For instance, the U5 snRNP 200 kDa helicase (SNRNP200; Brr2p in yeast) unwinds the initially extensively base-paired U4 and U6 snRNAs during spliceosome activation and releases U4 snRNA and all U4/U6-associated proteins, necessitating re-assembly of the U4/U6 di-snRNP and the U4/U6-U5 tri-snRNP after splicing. SNRNP200 comprises an auto-regulatory N-terminal region (residues 1–394), followed by a helicase region (residues 395–2129; SNRNP200HR) composed of tandem helicase cassettes (N-/C-terminal cassette, NC/CC). Both helicase cassettes comprise dual RecA-like NTPase domains, a winged helix (WH) domain, a helical bundle (HB) domain, a helix-loop-helix (HLH) domain and an immunoglobulin-like (IG) domain. Only the N-terminal cassette (residues 395–1324; SNRNP200NC) is an active ATPase/RNA helicase, while the C-terminal cassette (residues 1282–2136; SNRNP200CC) is catalytically inactive and serves as an intra-molecular regulator of the NC helicase activity.

We have previously characterized the interaction of SNRNP200 with two splicing factors that are also largely intrinsically disordered, FBP21 and C9ORF78 (34,35). FBP21 enters the spliceosome during formation of the pre-catalytic B complex together with seven additional B-specific proteins and leaves the spliceosome again during the following activation step, likely facilitating ordered transitions toward a catalytically competent spliceosome. Like TSSC4, both proteins also contact the SNRNP200 CC. Notably, the binding site of TSSC4 binding region 4 (residues 303–318) overlaps with a binding site of FBP21 and C9ORF78 regions at the Sec63 unit of the SNRNP200 CC. Moreover, all three proteins employ an F-R (F315-R316 in TSSC4; F8-R9 in C9ORF78) or L-R (L369-R370 in FBP21) motif to engage in similar contacts with the F1983, E1944 and E2119 residues of SNRNP200HR. This observation supports the idea that the SNRNP200 CC serves as a latching point for diverse intrinsically disordered proteins (IDPs) that either function during snRNP assembly (TSSC4) or during different stages of the splicing cycle (FBP21, C9ORF78). Mutually exclusive binding of the three proteins to SNRNP200 may serve to prevent premature interactions during U5 snRNP assembly (TSSC4) or support ordered recruitment of regulatory proteins during splicing (FBP21 and C9ORF78). Instead of full-length FBP21, we employed a C-terminal fragment (FBP21200–376) that encompasses the SNRNP200 CC-binding region. FBP21200–376 was fully displaced by GST-TSSC4 while, due to an excess of SNRNP200HR–C9ORF78 over GST–TSSC4 in case of the SNRNP200HR–C9ORF78/GST–TSSC4 mixture, a small amount of binary SNRNP200HR–C9ORF78 complex eluted from the SEC column in addition to SNRNP200HR–GST–TSSC4 and isolated C9ORF78. These observations indicate that TSSC4 exhibits a higher affinity to SNRNP200HR compared to FBP21200–376 or C9ORF78 and prevents binding of the latter two proteins.

> GAEFDLDQGGEALAPRQVLDLEDLVFTQGSHFMANKRCQLPDGSFRRQRKGYEEVHVPALKPKPFGSEEQLLPVEKLPKYAQAGFEGFKTLNRIQSKLYRAALETDENLLLCAPTGAGKTNVALMCMLREIGKHINMDGTINVDDFKIIYIAPMRSLVQEMVGSFGKRLATYGITVAELTGDHQLCKEEISATQIIVCTPEKWDIITRKGGERTYTQLVRLIILDEIHLLHDDRGPVLEALVARAIRNIEMTQEDVRLIGLSATLPNYEDVATFLRVDPAKGLFYFDNSFRPVPLEQTYVGITEKKAIKRFQIMNEIVYEKIMEHAGKNQVLVFVHSRKETGKTARAIRDMCLEKDTLGLFLREGSASTEVLRTEAEQCKNLELKDLLPYGFAIHHAGMTRVDRTLVEDLFADKHIQVLVSTATLAWGVNLPAHTVIIKGTQVYSPEKGRWTELGALDILQMLGRAGRPQYDTKGEGILITSHGELQYYLSLLNQQLPIESQMVSKLPDMLNAEIVLGNVQNAKDAVNWLGYAYLYIRMLRSPTLYGISHDDLKGDPLLDQRRLDLVHTAALMLDKNNLVKYDKKTGNFQVTELGRIASHYYITNDTVQTYNQLLKPTLSEIELFRVFSLSSEFKNITVREEEKLELQKLLERVPIPVKESIEEPSAKINVLLQAFISQLKLEGFALMADMVYVTQSAGRLMRAIFEIVLNRGWAQLTDKTLNLCKMIDKRMWQSMCPLRQFRKLPEEVVKKIEKKNFPFERLYDLNHNEIGELIRMPKMGKTIHKYVHLFPKLELSVHLQPITRSTLKVELTITPDFQWDEKVHGSSEAFWILVEDVDSEVILHHEYFLLKAKYAQDEHLITFFVPVFEPLPPQYFIRVVSDRWLSCETQLPVSFRHLILPEKYPPPTELLDLQPLPVSALRNSAFESLYQDKFPFFNPIQTQVFNTVYNSDDNVFVGAPTGSGKTICAEFAILRMLLQSSEGRCVYITPMEALAEQVYMDWYEKFQDRLNKKVVLLTGETSTDLKLLGKGNIIISTPEKWDILSRRWKQRKNVQNINLFVVDEVHLIGGENGPVLEVICSRMRYISSQIERPIRIVALSSSLSNAKDVAHWLGCSATSTFNFHPNVRPVPLELHIQGFNISHTQTRLLSMAKPVYHAITKHSPKKPVIVFVPSRKQTRLTAIDILTTCAADIQRQRFLHCTEKDLIPYLEKLSDSTLKETLLNGVGYLHEGLSPMERRLVEQLFSSGAIQVVVASRSLCWGMNVAAHLVIIMDTQYYNGKIHAYVDYPIYDVLQMVGHANRPLQDDEGRCVIMCQGSKKDFFKKFLYEPLPVESHLDHCMHDHFNAEIVTKTIENKQDAVDYLTWTFLYRRMTQNPNYYNLQGISHRHLSDHLSELVEQTLSDLEQSKCISIEDEMDVAPLNLGMIAAYYYINYTTIELFSMSLNAKTKVRGLIEIISNAAEYENIPIRHHEDNLLRQLAQKVPHKLNNPKFNDPHVKTNLLLQAHLSRMQLSAELQSDTEEILSKAIRLIQACVDVLSSNGWLSPALAAMELAQMVTQAMWSKDSYLKQLPHFTSEHIKRCTDKGVESVFDIMEMEDEERNALLQLTDSQIADVARFCNRYPNIELSYEVVDKDSIRSGGPVVVLVQLEREEEVTGPVIAPLFPQKREEGWWVVIGDAKSNSLISIKRLTLQQKAKVKLDFVAPATGAHNYTLYFMSDAYMGCDQEYKFSVDVKEA;> GAMAFNPHTSDLPSSKVNENSLGTLDESKSSDSHSDSDGEQEAEEGGVSTETEKPKIKFKEKNKNSDGGSDPETQKEKSIQKQNSLGSNEEKSKTLKKSNPYGEWQEIKQEVESHEEVDLELPSTENEYVSTSEADGGGEPKVVFKEKTVTSLGVMADGVAPVFKKRRTENGKSRNLRQRGDDQ>[2x]GAMEPLIDPYTQTNAVSYERFIRWYSKENHISATTEDLYNSLHGTYNNYKQDLYARTARSFVESHCDEAWFEDSYWVDESQGRVLEVSENEKSYRRALYDKFMDRLDAGYYDDFQLPTAE;>[2x]MEMPQLSKWNQDSRNDAMENTLLVSHVLPNISVAQIHNALDGISFVQHFSLSTINLIKNDERSLWVHFKAGTNMDGAKEAVDGIQLDSNFTIESENPKIPTHTHPIPIFEIASSEQTCKNLLEKLIRFIDRASTKYSLPNDAAQRIEDRLKTHASMKDDDDKPTNFHDIRLSDLYAEYLRQVATFDFWTSKEYESLIALLQDSPAGYSRKKFNPSKEVGQEENIWLSDLENNFACLLEPENVDIKAKGALPVEDFINNELDSVIMKEDEQKYRCHVGTCAKLFLGPEFVRKHINKKHKDWLDHIKKVAICLYGYVLDPCRAMDPKVVSSAWSHPQFEK;>KNEEDESNDSDKEDGEISEDD[2x]

The S. pombe MTREC complex and its human counterpart PAXT target specific and aberrant nuclear transcripts for degradation by the nuclear RNA exosome. The Red1 protein was shown to form a scaffold of the MTREC complex, interacting with multiple subunits and linking individual sub-modules together. The CBC and its partner ARS2 are implicated in fate determination of Pol II transcripts, including their processing, transport or degradation. The Red1-Mtl1 core also recruits the Cbc-Ars2 sub-module, which has been more extensively studied in human.

We also report a crystal structure of the Red1-Ars2 complex, which shows how the Ars2 C-terminal zinc-finger domain interacts with the conserved EDGEI motif of Red1. Only the minor dimeric version of Ars2 in complex with Red120–40 yielded single crystals, which diffracted to a 2.8 Å resolution. The S. pombe Ars2 structure consists of four defined domains, including a helical core with an inserted RNA recognition motif (RRM) and is flanked by two extended, mostly helical structures. Ars268–183,206–531 crystallized as a domain-swapped dimer, having the C-terminal leg segment exchanged between the two protomers. Red1 interacts with the Zn-finger domain of the Ars2 C-terminal leg, particularly with the surface formed by α14, β11 and β12. The peptide adopts a U-shape structure bent around the central G34 and establishes hydrophobic and charged contacts with Ars2, burying 300 Å2 of its surface. Red1 G34 and I36 together with aliphatic portions of D33 and E35 side chains pack against the Ars2 hydrophobic surface generated by K473, L484, F485, L486 and  F490. In addition, the three negatively charged residues E32, D33 and E35 make several hydrogen bonds and salt bridge interactions with Ars2 K483, K493, and H494. However, an important difference is the presence of a Zn atom coordinated by C476, C481, H494, and H499 in S. pombe, which is lacking in human ARS2, due to replacement of C481 by a serine. We generated structure-based mutations in the Zn-finger domain and Red1 peptide that abolish the binding in vitro and showed that Red1 E32R mutation is sufficient to disrupt binding with Ars2 in vivo.Transcription activator-like (TAL) effectors specifically bind to double stranded (ds) DNA through a central domain of tandem repeats. Each TAL effector (TALE) repeat comprises 33–35 amino acids and recognizes one specific DNA base through a highly variable residue at a fixed position in the repeat. The crystal structures of TAL effector (TALE) proteins bound to their respective target DNAs have revealed that the residue at position 13 is the only one directly involved in DNA base recognition, whereas the 12th residue stabilizes the proper loop conformation. dHax3, an engineered TALE protein, proved to be a useful scaffold for structural characterizations. We then present fifteen crystal structures of engineered dHax3 variants in complex with target DNA molecules, which elucidate the structural basis for the recognition of bases adenine (A) and guanine (G) by reported or uncharacterized TALE codes.

The structural observation suggests that Ile34 may not be a major contributor to the affinity of DNA binding by TALE repeats, consistent with the classification of NI as a “weak” TALE code. It also insinuates that base A may “tolerate” a wide range of amino acids at position 34 of a TALE repeat when there is no steric clash. To test this speculation, we generated dHax3 variants with the 34th residue on repeat 7 substituted with different amino acids. In total, we obtained nine high-quality structures that elucidate the accommodation of base A by Leu, Met, Cys, Pro, Trp, His, Thr, Asn, and Glu at the 34th position. Among these, the hydrophobic residues Leu, Met, Cys, and Pro all adopt conformations that do not clash with base A. As what happens to Ile34, there is no specific coordination found between these hydrophobic residues and base A. Trp, Thr, and His, in spite of the presence of polar groups, do not form H-bond with base A. They also appear to adopt conformations that simply avoid steric clash. These residues may all represent weak code, if they are used for base recognition.

>[2x]MQWSGARALEALLTVAGELRGPPLQLDTGQLLKIAKRGGVTAVEAVHAWRNALTGAPLNLTPEQVVAIASHDGGKQALETVQRLLPVLCQAHGLTPQQVVAIASHDGGKQALETVQRLLPVLCQAHGLTPEQVVAIASHDGGKQALETVQALLPVLCQAHGLTPEQVVAIASNGGGKQALETVQRLLPVLCQAHGLTPQQVVAIASNGGGKQALETVQRLLPVLCQAHGLTPQQVVAIASNGGGKQALETVQRLLPVLCQAHGLTPQQVVAIASNLGGKQALETVQRLLPVLCQAHGLTPQQVVAIASNGGGKQALETVQRLLPVLCQAHGLTPQQVVAIASHDGGKQALETVQRLLPVLCQAHGLTPEQVVAIASNGGGKQALETVQRLLPVLCQAHGLTPEQVVAIASHDGGKQALETVQRLLPVLCQAHGLTPQQVVAIASNGGGRPALESIVAQLSRPDPALAALTNDHLVALACLGGRPALDAVKKLEHHHHHH>[2x]GRKEPEIITVTLKKQNGMGLSIVAAKGAGQDKLGIYVKSVVKGGAADV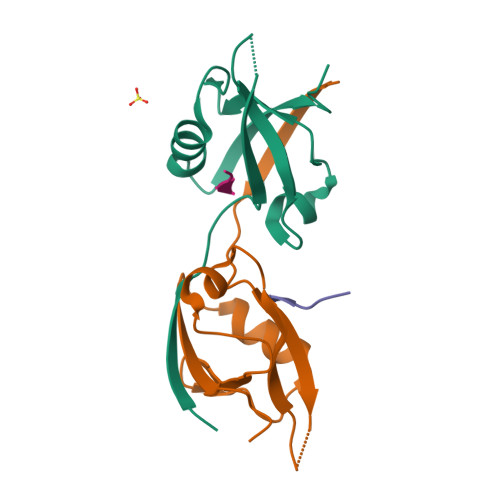DGRLAAGDQLLSVDGRSLVGLSQERAAELMTRTSSVVTLEVAKQGAIYH;>NLNSSRVPDLLV[2x]6-((2-chlorophenyl)thio)-[1,2,4]triazolo[4,3-b]pyridazin-3(2H)-one 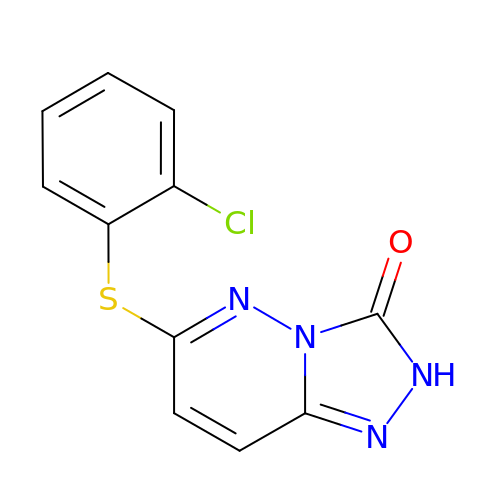| C11 H7 Cl N4 O S | IOETYCRGZYHINY-UHFFFAOYSA-N> GPMNKILGFSKYWVEINNWILPTLDHIGLTLWGMIKKHASEYRGIRYSLEKFGELKIIHYIGSRASHDLGKTFIGESVLSKENNKIVKEYSWPEIKKVLRKIFLDNGISSDTIDQYFIAIRRIIRPSRSDRFFLFRLAEYRKYENPVKYDQVRDIISHIT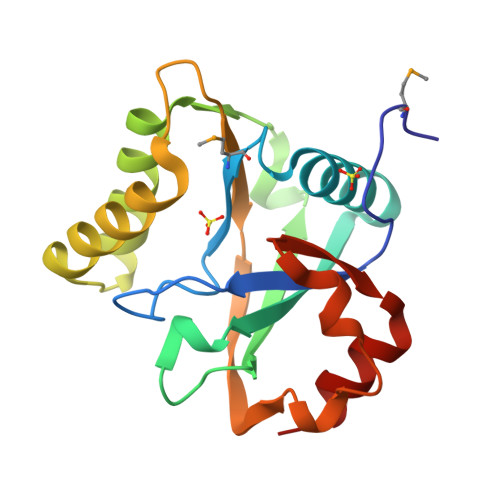WTGRYLVPIRPEDYEAIHSRG> MSIQAFVFCGKGSNLAPFTQPDFPFQTQNKDSTAATSGDKLNELVNSALDSTVINEFMQHSTRLPKALLPIGNRPMIEYVLDWCDQADFKEISVVAPVDEIELIESGLTSFLSLRKQQFELIYKALSNSNHSHHLQDPKKINFIPSKANSTGESLQKELLPRINGDFVILPCDFVTDIPPQVLVDQFRNRDDNNLAMTIYYKNSLDSSIDKKQQQKQKQQQFFTVYSENEDSERQPILLDVYSQRDVTKTKYLQIRSHLLWNYPNLTVSTKLLNSFIYFCSFELCQLLKLGPQSMSRQASFKDPFTGNQQQQNPPTTDDDEDRNHDDDDDYKPSATSIQPTYFKKKNDLILDPINCNKSLSKVFRDLSRRSWQHSKPREPIGIFILPNETLFIRANNLNAYMDANR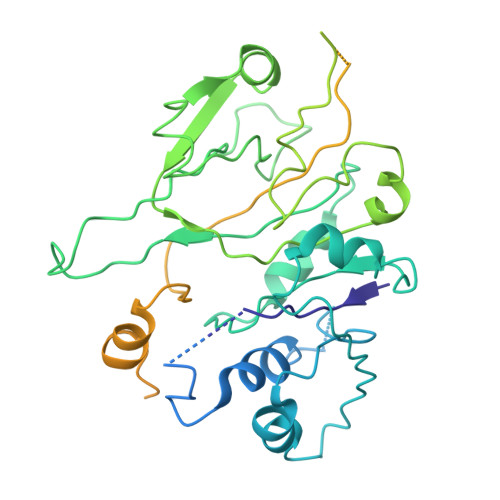FVLKIKSQTMFTKNIQIQSAAIGADAIVDPKCQISAHSNVKMSVLGTQANIGSRCRVAGSLLFPGVHLGDEVILENCIIGPMAKIGSKCKLSNCYIEGHYVVEPKNNFKGETLANVYLDEDEEDELIYDDSVIAGESEIAEETDSDDRSDEDSDDSEYTDEYEYEDDGLFER 4-{[(3-Chloro-6,7,10,11-tetrahydro-9-methyl-7,11-methanocycloocta[b]quinolin-12-yl)amino]methyl}-N-(4-hydroxy-3-methoxybenzyl)benzamide 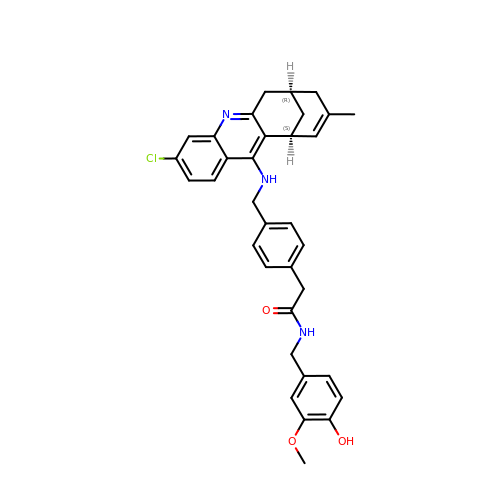| C34 H34 Cl N3 O3 | BWBXSBFNPJZWIY-LOSJGSFVSA-N>SNATYKVDGKGTYYKAESASFTANYDIKTRLNGPFRSNPQSGVLHPGQTIKYDTVMKQDGHVWVVYTGYSGKRIYLPVRT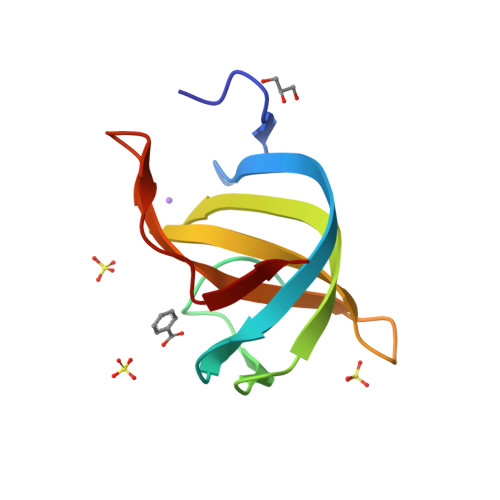WDKNSNTLGPLWGIIN[2x]>AQPDIKFASKEYGVTIGESRIIYPLDAAGVMVSVKNTQDYPVLIQSRIYDENKEKESEDPFVVTPPLFRLDAKQQNSLRIAQAGGVFPRDKESLKWLCVKGIPPKDE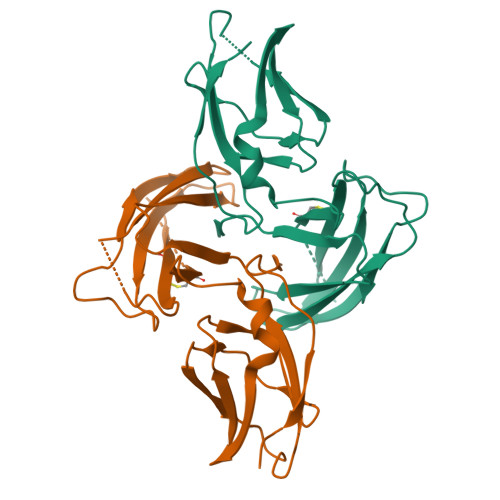DIWVDVQFAINNCIKLLVRPNELKGTPIQFAENLSWKVDGGKLIAENPSPFYMNIGELTFGGKSIPSHYIPPKSTWAFDLPKGLAGARNVSWRIINDQGGLDRLYSKNVTL[2x]> AEVKACSSELESLEMELRQQILVNIGKILQDQPSMEALEASLGQGLCSGGQVEPLDGPAGCILECLVLDSGELVPELAAPIFYLLGALAVL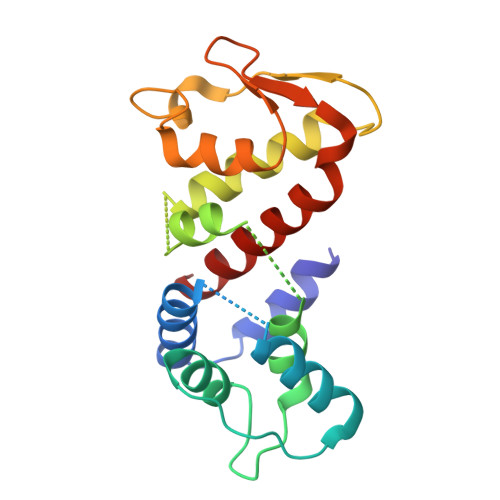SETQQQLLAKALETTVLSKQLELVKHVLEQSTPWQEQSSVSLPTVLLGDCWDEKNPTWVLLEECGLRLQVESPQVHWEPTSLIPTSALYASLFLLSSLGQ> MASIPSAAPSWRKMQIPRPLQRLFDYFPLRIYEPNELPERSQQLTSGDLP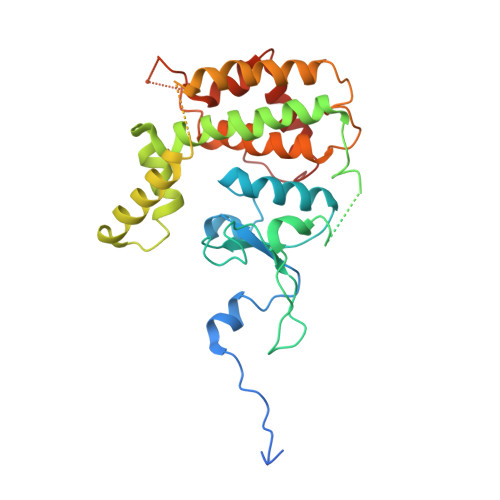TLYVFSTDSDARLGLPSFNPGCLKWQTLLRLANLDFRILPSTNHSSPTGSLPFLLPPRTSPTASPAPIPASGLLSFARKNPWRPGKAADLDLGHLDADLPPRAQAYLALITHSLRNAWLCALYLDPTHDALLRRLYVDPASSSRAVRAALLHQLRRAAAEQVATASSGGGKIVSLAPVDSADGIDEEAVYRSARDALDALASLLRESETAWFGTERPGSFDAALFSYTHLMVEYMSEEEDTESAKGRVSLGRMVKEAGNGELAEHRERMLGVAWPEWDGYRR> ARKIPLDLPGTRILNGANWANNSATENLATNSGTLIIFDQSTPGQDADRWLIHNYLDGYKIFNMGSNNWASVSRGNTVLGVSEFDGQTCKWSIEY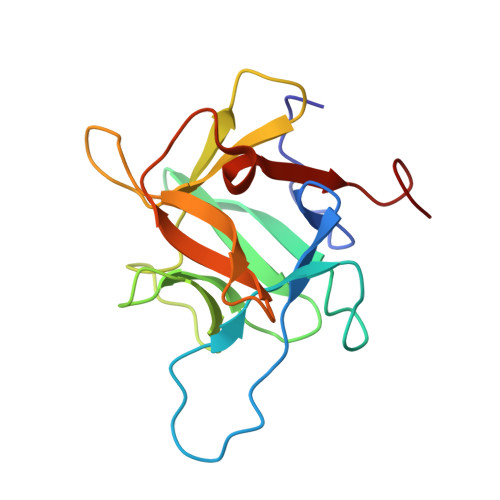SGNGEEFWIRVPREGGGGAVWTIKPASSQGPTTVFLDLLKETDPNQRIKFAVENLYFQ>[2x]MEKVKVKNPIVELDGDEMARVMWKMIKEKLILPYLDIQLVYFDLGIKKRDETDDQITIEAAKAIKKYGVGVKCATITPDAERVKEYNLKKAWKSPNATIRAYLDGTVFRKPIMVKNVPPLVKRWKKPIIIGRHAYGDIYNAVEAKVEGPAEVELVVRNKENKTLLVHKFEGNGVVMAMHNLEKSIRSFAQSCINYAISEKVDIWFATKDTISKVYH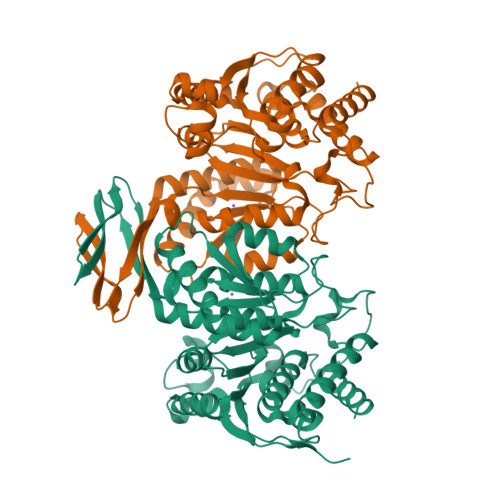AYFKDIFQEEVDKRKEELEKAGVNYRYMLIDDAAAQILRSEGGMLWACMNYEGDIMSDMIASGFGSLGLMTSVLVSPDGVYEFEAAHGTVRRHYYRYLKGEKTSTNPTASIFAWTGAIRKRGELDGTPEVCEFADKLEKAVINTIESGVITKDLQPFTEPPIDKYVTLEEFIDEVKKNLEKLL> MGSSHHHHHHSSGLVPRSHMEQLEEDCVHRYGVNAFVLYRLPVVKEGMVVGIVGPNGTGKSTAVKILAGQLIPNLCGDNDSWDGVIRAFRGNELQNYFEKLKNGEIRPVVKPQYVDLIPKAVKGKVIELLKKAD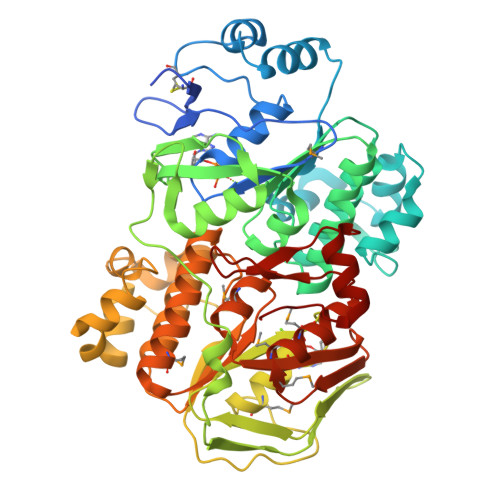ETGKLEEVVKALELENVLEREIQHLSGGELQRVAIAAALLRNATFYFFDEPSSYLDIRQRLNAARAIRRLSEEGKSVLVVEHDLAVLDYLSDIIHVVYGEPGVYGIFSQPKGTRNGINEFLRGYLKDENVRFRPYEIKFTKTGERVEIERETLVTYPRLVKDYGSFRLEVEPGEIKKGEVIGIVGPNGIGKTTFVKMLAGVEEPTEGKIEWDLTVAYKPQYIKADYEGTVYELLSKIDASKLNSNFYKTELLKPLGIIDLYDREVNELSGGELQRVAIAATLLRDADIYLLDEPSAYLDVEQRLAVSRAIRHLMEKNEKTALVVEHDVLMIDYVSDRLMVFEGEPGKYGRALPPMGMREGMNRFLASIGITFRRDPDTGRPRANKEGSVKDREQKEKGEYYYIA>MRSSHHHHHHSSGLVPRGSHMESKKDDTDLKLVSHNVYMLSTVLYPNWGQYKRADLIGQSSYIKNNDVVIFNEAFDNGASDKLLSNVKKEYPYQTPVLGRSQSGWDKTEGSYSSTVAEDGGVAIVSKYPIKEKIQHVFKSGCGFDNDSNKGFVYTKIEKNGKNVHVIGTHTQSEDSRCGAGHDRKIRAEQMKEISDFVKKKNIPKDETVYIGGDLNVNKGTPEFKDMLKNLNVNDVLYAGHNSTWDPQSNSIAKYNYPNGKPEH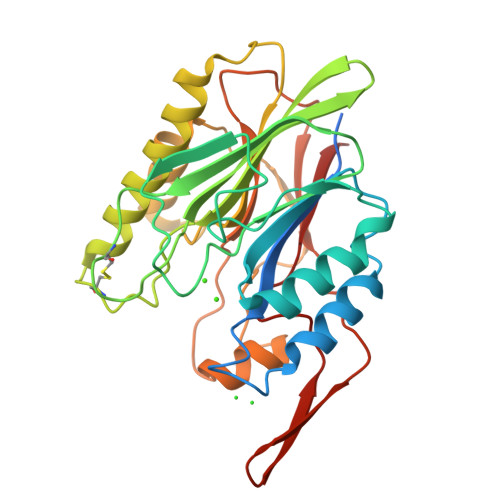LDYIFTDKDHKQPKQLVNEVVTEKPKPWDVYAAAYYYVYNDFSDHYPIKAYSK[2x]>GGSRSSSHSSRRAKSVEDDAEGHLIYHVGDWLQERYEIVSTLGEGTFGRVVQCVDHRRGGARVALKIIKNVEKYKEAARLEINVLEKINEKDPDNKNLCVQMFDWFDYHGHMCISFELLGLSTFDFLKDNNYLPYPIHQVRHMAFQLCQAVKFLHDNKLTHTDLKPENILFVNSDYELTYNLEKKRDERSVKSTAVRVVDFGSATFDHEHHSTIVSTRHYRAPEVILELGWSQPCDVWSIGCIIFEYYVGFTLFQTHDNREHLAMMERILGPIPSRMIRKTRKQKYFYRGRLDWDENTSAGRYVRENCKPLRRYLTSEAEEHHQLFDLIESMLEYEP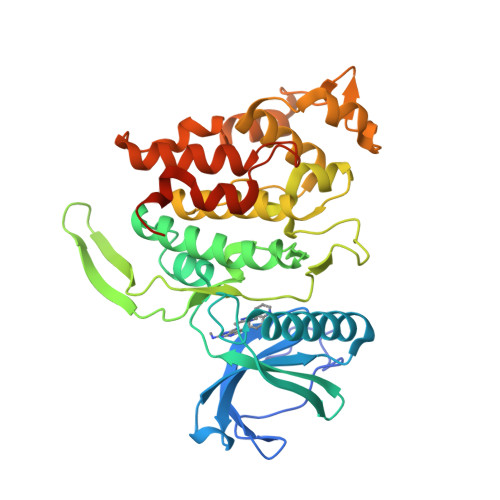AKRLTLGEALQHPFFARLRAEPPNKLWDSSRD[2x]> GSMSWRHIRAEGLDSSYTVLFGKAEADEIFQELEKEVEYFTGALARVQVFGKWHSVPRKQATYGDAGLTYTFSGLTLSPKPWIPVLERIRDHVSGVTGQTFNFVLINRYKDGSDHICEHRDDERDLAPGSPIASVSFGASRDFVFR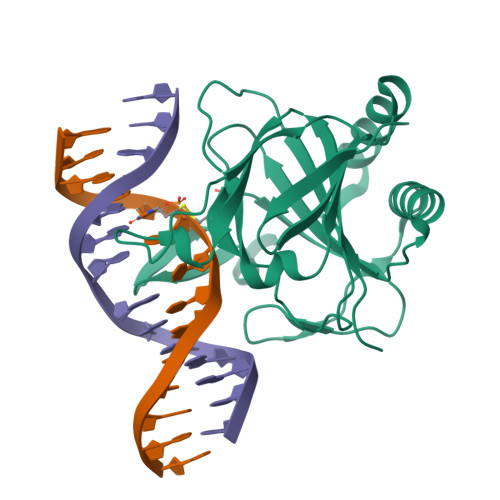HKDSRGKSPSRRVAVVRLPLAHGSLLMMNHPTNTHWYHSLPVRKKVLAPRVNLTFRKILLTKK>[2x]MGSHHHHHHSQDSVTIFILSVIHVKPPFKLKRKFQNNPHYEKEMRRQLKMQEDGINKLTVFEWLTNRKTFREKGRLSSQTAQNDARDAYKRRKMFDYMLLSAENFKYDEITKKVEDELSSLAALHNPDQIAGGNFDDVTAMGDKRINSSIGSQWGTKDKGRAQNLEDELLKVLEGPPKIDEEQQKYIKMNVIFAEDLEIIK;>[2x]MYEMFLFNSVNSKITQNVNEEFILKYSDYSCEQLNSLWKEVGLGSYYNGLFKIIEPNDLKDIINQCYIMDDDESLLPFMCTAFGDVFAYVKNKRFGNYVVFLNIRYGTSLIIPDNFVAIFNKVIPNQSFLKGWFDLENYAFVKEKIGEIDFDECYGYFPTLSMGGNESIDNISIVKMIPYIDMNVQMIDVFERADKHHHHHH

We identify a horizontally transferred T6SS with Ntox15 family nuclease effector (Tde1) that mediates interbacterial antagonism among Bacteroidales, including several derived from a single human donor. Effectors with novel toxin 15 (Ntox15) DNAse domains, also known as toxin_43 domains, degrade recipient genomic DNA. Cognate immunity proteins are encoded adjacent to T6SS effectors and neutralize their activity to prevent intoxication of self and kin. Crystallographic snapshots of isolated Tde1, the Tde1/Tdi1 complex, and homologs from Phocaeicola vulgatus (Tde2/Tdi2) illustrate a conserved mechanism of immunity inserting into the central core of Tde, splitting the nuclease fold into two subdomains.

Orphan immunity proteins co-expressed with the P. vulgatus dnLKV7 homolog Tde2tox in E. coli also formed a stable 1:1 complex, as detected with analytical gel filtration chromatography. We therefore obtained crystal structures of the Tde1 Ntox15 domain in complex with Tdi1, as well as a homologous complex from P. vulgatus dnLKV7, Tde2tox and Tdi2. The Tdetox/Tdi complex homologs exhibit very similar structure despite 51% sequence identity between the Ntox15 domains, indicating a conserved mode of effector–immunity interaction. When bound to immunity proteins, Tde1tox and Tde2tox split into two subdomains. Forty percent (17 of 43) of immunity-contacting Tde1/2tox residues in the effector immunity structures form part of the central core in the globular Ntox15 domain alone structure, and many of these are highly conserved. Tdi1 and Tdi2 form extensive contacts with the conserved central cores of their Tdetox counterparts. We conclude that Tdi immunity proteins induce a marked conformational shift in Tde effectors, driving a division into two subdomains with disruption of the enzymatic active site and DNA binding motif.> SVVKVSLTHSASRMRVPEKRYGLAQTIESIKENVFTHFATPPEYMQLQLIDDRGITIEKNMANDKQLGYYQCRDEFVIHVVDLQPS

Five tubulin-binding cofactors (TBCs) are implicated in late-stage tubulin folding and heterodimer assembly 1,5–10. TBC-B and TBC-E are implicated in binding α-tubulin, whereas TBC-A and TBC-D interact with β-tubulin. TBC-B comprises an N-terminal ubiquitin-like (Ubl) domain and a C-terminal cytoskeleton-associated protein with glycine-rich segment (CAP-Gly) domain.

Limited proteolysis produced two polypeptides, one of which, the Ubl domain, gave highly ordered crystals, and the structure was solved with anomalous dispersion methods 14. The N-terminal Ubl domain of TbTBC-B crystallized in the tetragonal space group P41212 with a single polypeptide in the asymmetric unit. The Ubl domain is a small globular entity consisting of a mixed four-strand β-sheet that forms a concave groove in which a single α-helix is placed. This is an example of a β-grasp fold, a common structure involved in protein–protein interactions 5–11. A pronounced hydrophobic core is present, formed mainly by aliphatic side chains. The residues involved, which have < 10% solvent-accessible surface area, include Val4, Val6, Leu8, Tyr22, Ile28, Ile31, Val35, Thr41, Met46, Leu48, Leu50, Met62, Leu68, Cys73, Ile79, and Val81 (not shown). These core residues are, in general, conserved among the TBC-B family of proteins. The surface residues are more variable, perhaps indicative of a module that does not interact directly with α-tubulin. Intriguingly, and despite only low sequence conservation, the Ubl domain of TbTBC-B contains two lysines (Lys34 and Lys62), which correspond to Lys27 and Lys48 of ubiquitin, and a structural overlay reveals strong structural similarity in terms of the positioning of these residues. A striking similarity is observed in the spatial location of two functionally important lysines in ubiquitin, and strongly supports a biological function for the Ubl domain, and by implication for TBC-B. Through reversible post-translational modification, TBC-B can influence aspects of tubulin biology in a proteasome-dependent manner.Recently, two group A flavoprotein monooxygenases (FPMOs) (GrhO5 and GrhO6) and a flavoprotein oxidase (GrhO1) were shown to mediate the drastic remodeling of the 3 backbone and subsequent spiroketal pharmacophore formation. First, GrhO5 generates a ‐spiroketal moiety as part of the advanced intermediate dihydrolenticulone (4), which entails the rupture of three C−C bonds and a CO2 elimination step. The functional homolog RubL from rubromycin biosynthesis was shown to catalyze the same reaction sequence, pointing toward a universal strategy for spiroketal formation in the rubromycin family. In this work, the combined crystal structures of GrhO5 and RubL suggest three interconvertible catalytically relevant conformers, hereafter referred to as the “acceptor state” (FADox in OUT; accepts substrate, no reaction with NADPH), “reducible state” (FADox in OUT with bound substrate; reducible by NADPH) and the “catalytic state” (FADred in IN with bound substrate; reacts with O2 for hydroxylation).

Hence, crystallization screens under high‐salt concentrations were conducted, in which only RubL crystals formed in presence of shunt product 7 that diffracted to a resolution of 1.6 Å. Indeed, a Cl− was found coordinated between the C4a‐position of the FAD cofactor and the protein backbone including P316 (distance of 3.5–4 Å from the proline carbonyl to Cl−), which is conserved in the majority of group A FPMOs. Notably, although the active site was partially occupied, clear electron density for the shunt‐product was not observed. However, the FAD cofactor shifted and adopts the “IN”‐conformation, which is stabilized by several hydrogen‐bonds formed between the heteroatoms of the isoalloxazine ring and the protein backbone as well as amino acid side chains. Strikingly, several active site residues have a different rotameric state compared to native and 3‐soaked GrhO5 with F287 and W289 now stabilizing the FAD conformation by direct T‐shaped (W289 to FAD) and indirect (F287 to W289) π‐π interactions (see Figure S7 for all interactions). At the same time, rotation of these amino acid side‐chains results in the opening of the NADPH‐entry site, which may be beneficial for the efficient release of NADP+. Notably, co‐crystallization of RubL with 7 apparently also caused a loop ordering (residues 90–110), which resulted in the closure of the substrate entry site and a more confined reaction chamber. Overall, these changes lead to the catalytic state of the enzyme. The observed Cl− adjacent to the FAD cofactor indicates this site, which is likely optimized to trap the transient superoxide long enough to allow spin inversion and collapse of the radicals to the FADC4aOOH (step IV). In this process, the backbone carbonyl group of the highly conserved proline of group A FPMOs (P316 in RubL) may function as an H‐bond acceptor to stabilize and position the FADC4aOOH intermediate to ensure regiospecific hydroxylation.

> MTSASEPSGPSGSAPVLIVGGSLVGLSTAVFLARHGVRCTLVERHPGTSVHPRAVGYYPRTGELLRQAGVEDAAVREASGFATHRTRAGVTSLAGEVLFSKEELEGDDDLGDLTPSRLLLLPQDRLEPLLRDRAVELGADLRFGTELVSFAEDPEGVTAVLDDGTGGTRTFRSSYLVACDGPRSTVREALKVPRQGRGVLSRHVSIAFGADLRPVLGDRRYSVVHVKNPQVTGILVHDDTLTGGTLIVGYRPEDGESLEDFTDDRCAELVGAAVGAPGVEVTIRSRFPWDMAEQVAESFVHGRVLLAGDAAHVVPPTGGYGANTGIADAHNLAWKLALVAAGVAGPGLVETYDAERRPVAVYTAEQGSLQLALRSGTATPEQQAAVADAVTVTSGQAYRSTAVVGEPDGADLPVASDPRELRGAPGTRAPYVELLRGGETVSTLDLFGRDFVLLTGEHGREWISAAVSASAGLGLKITARRVVPGTDAGAGTLADPDGDWSERYGGLRPEGAVLVRPDGVVAWRSPGADPGGEESAVLAAVLRSVLARESRTGGK>[2x]TPEMPVLENRAAQGDITAPGGARRLTGDQTAALRDSLSDKPAKNIILLIGDGMGDSEITAARNYAEGAGGFFKGIDALPLTGQYTHYALNKKTGKPDYVTDGAASATAWSTGVKTYNGALGVDIHEKDHPTILEMAKAAGLATGNVSTAELQDATPAALVAHVTSRKCYGPSA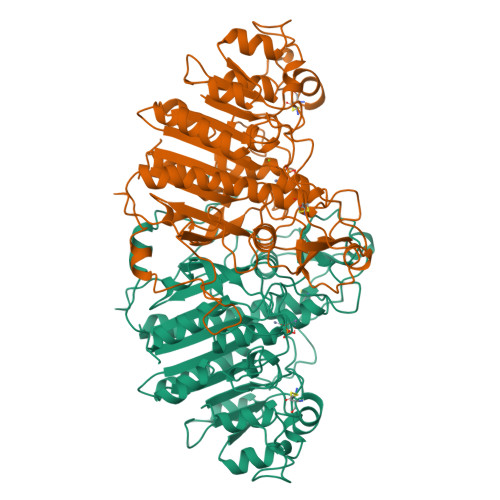TSEKCPGNALEKGGKGSITEQLLNARADVTLGGGAKTFAETATAGEWQGKTLREQAQARGYQLVSDAASLNSVTEANQQKPLLGLFADGNMPVRWLGPKATYHGNIDKPAVTCTPNPQRNDSVPTLAQMTDKAIELLSKNEKGFFLQVEGASIDKQDHAANPCGQIGETVDLDEAVQRALEFAKKEGNTLVIVTADHAHASQIVAPDTKAPGLTQALNTKDGAVMVMSYGNSEEDSQEHTGSQLRIAAYGPHAANVVGLTDQTDLFYTMKAALGLK> FPTIPLSRLFDNAMLRAHRLHQLAFDTYQEFEEAYIPKEQKYSFLQNPQTSLCFSESIPTPSNREETQQKSNLELLRISLLLIQSWLEPVQFLRSVFANSL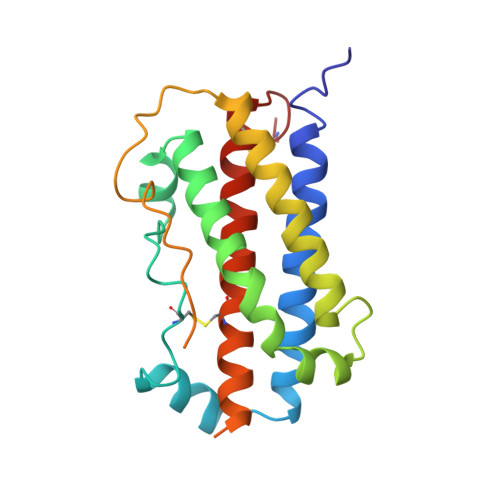VYGASDSNVYDLLKDLEEGIQTLMGRLEDGSPRTGQIFKQTYSKFDTNSHNDDALLKNYGLLYCFRKDMDKVETFLRIVQCRSVEGSCG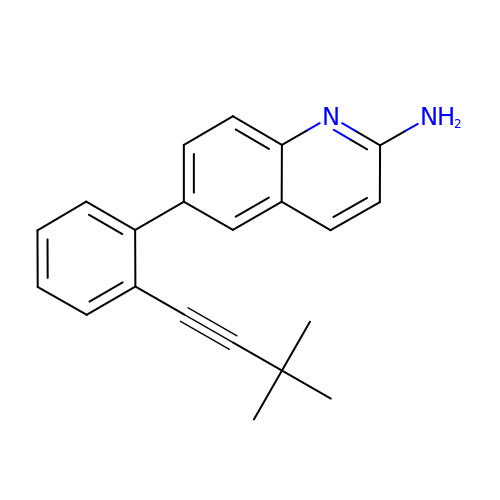6-[2-(3,3-dimethylbut-1-yn-1-yl)phenyl]quinolin-2-amine | C21 H20 N2 | IFUYBWIZKMAADM-UHFFFAOYSA-N>[4x]MKFTVEREHLLKPLQQVSGPLGGRPTLPILGNLLLQVADGTLSLTGTDLEMEMIARVTLSQPHEAGATTVPARKFFDICRGLPEGAEIAVQLEGDRMLVRSGRSRFSLSTLPAADFPNLDDWQSEVEFTLPQATMKRLIEATQFSMAHQDVRYYLNGMLFETEGEELR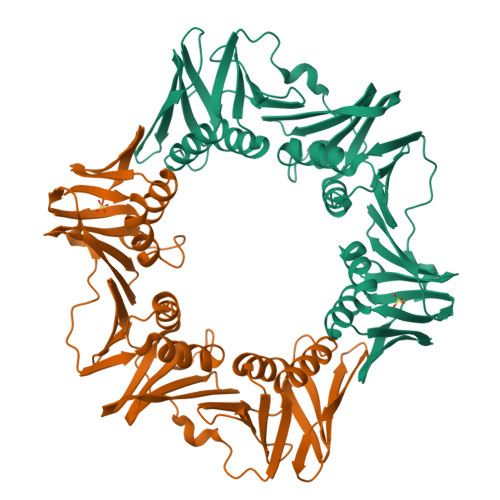TVATDGHRLAVCSMPIGDSLPNHSVIVPRKGVIELMRMLDGGDTPLRVQIGSNNIRAHVGDFVFTSKLVDGRFPDYRRVLPKNPDKTLEAGCDSLKQAFARAAILSNEKFRGVRLYVSENQIKITANNPEQEEAEEILDVTYAGTEMEIGFNVSYVLDVLNALKCENVRILLTDSVSSVQIEDAASQSAAYVVMPMRL SSNA1 is a fibrillar protein involved in dynamic microtubule remodeling, including nucleation, co-polymerization, and microtubule branching. Although SSNA1 is only a small 14 kDa protein mostly comprised of a coiled-coil domain, it grows into long fibrils through a self-assembly process. In vitro studies have characterized SSNA1 as a microtubule-binding protein that facilitates the nucleation of microtubules. Although its precise role has been enigmatic, SSNA1 is essential for cell integrity, and it is highly conserved across eukaryotic species from algae to humans.

We however note that three point mutations (R18E/R20E/Q98E, 3E) were introduced to facilitate structure determination, as the wild-type C. elegans SSNA-1 formed bundled filaments unsuitable for analysis. Cryo-EM analysis of SSNA-1(3E) revealed the presence of 8 parallel fibrils assembled into filaments with C8 symmetry with a periodicity of 112 Å, which was also validated by the averaged power spectrum of the aligned filaments. The outer and inner diameters of the filaments were 90 Å and 55 Å, respectively. Within each fibril of the filament, individual protomers were arranged in double-stranded coiled-coils and longitudinally connected to adjacent coiled-coil units via triple-stranded helical junctions. Our model building revealed that the coiled-coil within each protomer unit (CC1-a1 and CC1-a2) assembles in an antiparallel manner, spanning residues 9-105, unlike the previous publications following a conventional assumption that the coiled-coil running in parallel with little structural information. Interestingly, the C-terminal helix of each protomer unit forms an overhang and reaches into the adjacent double-stranded helical arrangement creating a triple-stranded junction. The overhanging C-terminus of the first coiled-coil (CC1-a1) forms a triple-stranded helix with two alpha helices of the second coiled-coil (CC2). The key residues in the triple-helical junction are the N-terminal residues Y15, R18E, L19 of one strand and the C-terminal residues L89, Y97, Y105 of the partnering coiled-coil helix. The electrostatic surface potential analysis of the 3E mutant shows the presence of negatively charged patches, primarily attributed to the specific 3E mutations (R18E/R20E/Q98E) and the neighbouring charged residues within the three-stranded junctions. While residues R18E and R20E were oriented towards the inner lumen, residue Q98E was located at the interfilamentous interfaces. These negative charges likely act as a repulsive force to separate the SSNA-1 bundles into 8-stranded filaments, making it amenable to our structural analysis.

>[32x]MGKHHHHHHGSLEVLFQGPMSSRSTGSFDEISQYIQELEEERRLTESSIRKMEKEKSDLNEKIDELTTRKCSVDARLQAENERAERQDRGLKEAETTYAKLVESQKTLVDFVRKEYEDTKHQKY> GPDSMKETPLSNCERRFLLRAIEEKKRLDGRQTYDYRNIRISFGTDYGCCIVELGKTRVLGQVSCELVSPKLNRATEGILFFNLELSQMAAPAFEPGRQSDLLVKLNRLMERCLRNSKCIDTESLCVVAGEKVWQIRVDLHLLNHDGNIIDAASIAAIVALCHFRRPDVSVQGDEVTLYTPEERDPVPLSIHHMPICVSFAFFQQGTYLLVDPNEREERVMDGLLVIAMNKHREICTIQSSGGIMLLKDQVLRCSKIAGVKVAEITELILKALENDQKVRKEGGKFGFAESIANQRITAFKMEKAPIDTSDVEEKAEEIIAEAEPPSEVVSTPVLWTPGTAQ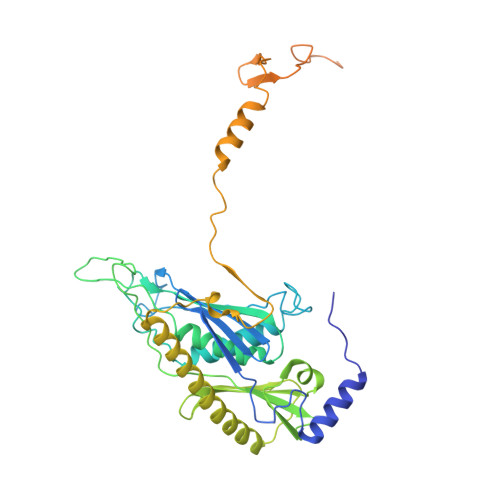IGEGVENSWGDLEDSEKEDDEGGGDQAIILDGIKMDTGVEVSDIGSQDAPIILSDSEEEEMIILEPDKNPKKIRTQTTSAKQEKAPSKKPVKRRKKKRAAN>[2x]STAGKVIKCKAAVLWEEKKPFSIEE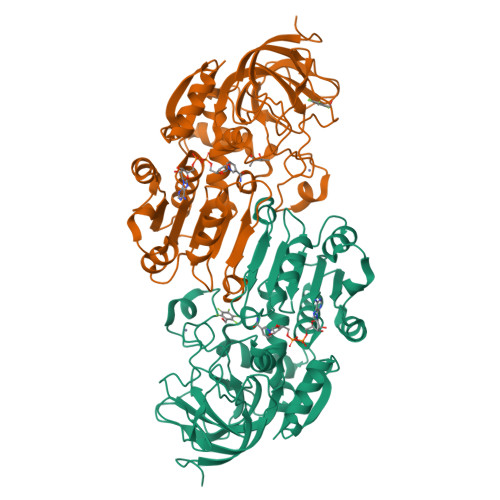VEVAPPKAHEVRIKMVATGICRSDDHVVSGTLVTPLPVIAGHEAAGIVESIGEGVTTVRPGDKVIPLATPQCGKCRVCKHPEGNFCLKNDLSMPRGTMQDGTSRFTCRGKPIHHFLGTSTFSQYTVVDEISVAKIDAASPLEKVCLIGCGFSTGYGSAVKVAKVTQGSTCAVFGLGGVGLSVIMGCKAAGAARIIGVDINKDKFAKAKEVGATECVNPQDYKKPIQEVLTEMSNGGVDFSFEVIGRLDTMVTALSCCQEAYGVSVIVGVPPDSQNLSMNPMLLLSGRTWKGAIFGGFKSKDSVPKLVADFMAKKFALDPLITHVLPFEKINEGFDLLRSGESIRTILTF> MSEMSYLEKLLDGVEVEWLPLGEITKYEQPTKYLVKAKDYHDTYTI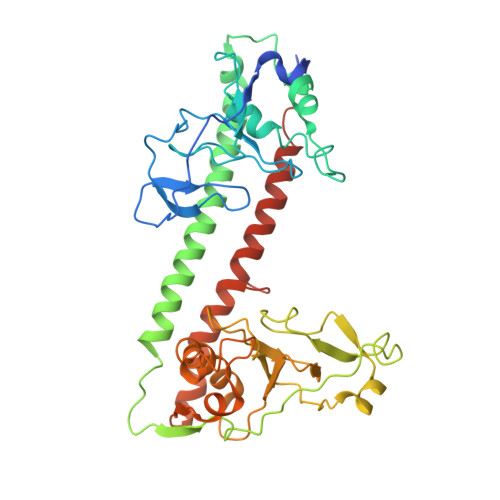PVLTAGKTFILGYTNETHGIYQASKAPVIIFDDFTTANKWVDFDFKAKSSAMKMVTSCDDNKTLLKYVYYWLNTLPSEFAEGDHKRQWISNYSQKKIPIPCPDNPEKSLAIQSEIVRILDKFTALTAELTAELNMRKKQYNYYRDQLLSFKEGEVEWKTLGEIGKWYGGGTPSKNKIEFWENGSIPWISPKDMGRTLVDSSEDYITEEAVLHSSTKLIPANSIAIVVRSSILDKVLPSALIKVPATLNQDMKAVIPHENILVKYIYHMIGSRGSDILRAAKKTGGSVASIDSKKLFSFKIPVPNINEQQRIVEILDKFDTLTNSITEGLPREIELRQKQYEYYRDLLFSFPKPETVSN> KENALLRYLLDK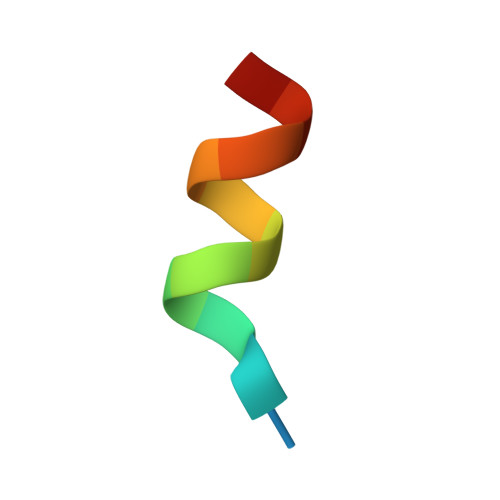D> KVFERCELARTLKRLGMDGYRGISLANWMCLAKWESGYNTRATNYNAGDRSTDYGIFQINSRYWCNDGKTPGAVNAAHLSCSALLQDNIADAVAAAKRV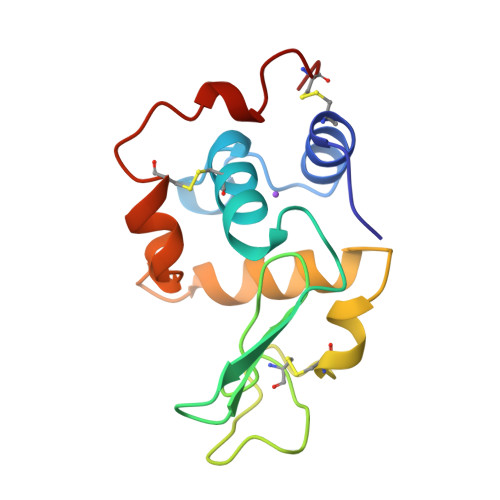VRDPQGVRAWVAWRNRCQNRDVRQYVQGCGV>GSMGLYFSSLDSSIDILQKRAQELIENINKSRQKDHALMTNFRNSLKTKVSDLTEKLEERIYQIYNDHNKIIQEKLQEFTQKMAKISHLETELKQVCHSVETVYKDLCLQPE[2x];>GSMGKDEALEKDLNDVSKEINLML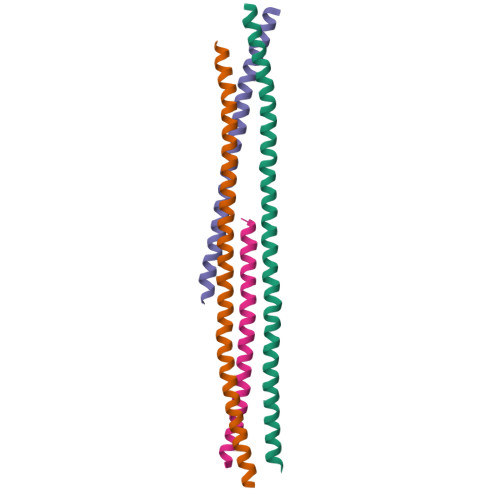STYAKLLSERAAVDASYIDEIDELFKEANAIENFLIQKREFLRQR[2x]> SAPANAVAADNATAIALKYNQDATKSERVAAARPGLPPEEQHCADCQFMQADAAGATDEWKGCQLFPGKLIN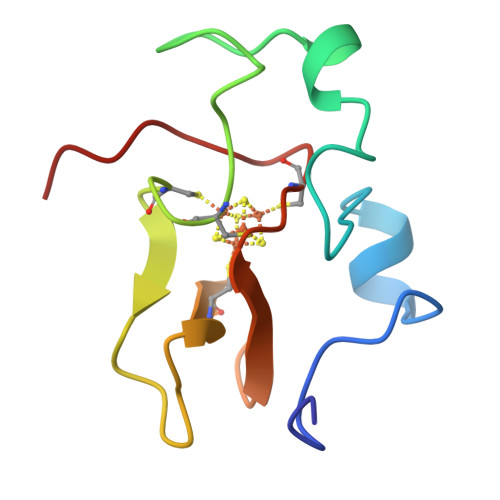VNGWCASWTLKAG> NECLGTIGPVTPLDASDFALDIRMPGVTPKESDTYFCMSMRLPVDEEAFVIDFKPRASMDTVHAMLLFGCNMPSSTGSYWFCDEGTCTDKANILYAWARNAPPTRLPKGVGFRVGGETGSKYFVLQVHYGDISAFRDNHKDCSGVSVHLTRVPQPLIAGMYLMMSVDTVIPPGEKVVNADISCQYKMYPMHVFAYRVHTHHLGKVVSGYRVRNGQWTLIGRQNPQLPQAFYPVEHPVDVTFGDILAARCVFTGEGRTEATHIGGTSSDEMCNLYIMYYMEAKYALSFMTCTKNVAPDMFRTIPAEANIPIPV

The two recently opened beamlines for macromolecular crystallography at NSLS-II have launched the microcrystallography field into new territory, with flux densities up to two orders of magnitude brighter than those previously available. In this study, we highlight the capabilities of the AMX and FMX beamlines at NSLS-II by describing structure determination from single crystal vector data collection and two methods for multicrystal data collection. The advent of next generation synchrotron beamlines has necessitated the development of new strategies to fully benefit from the increased beam intensity and smaller beam sizes while minimizing radiation damage. The high dose rates, in conjunction with the newly developed ultrafast raster scanning goniometer brings formerly time-consuming serial crystallography measurements into the minutes range. These new opportunities mean that inhomogeneous large crystals can now deliver high quality data collected from their best volume, and crystals as small as 5 to 10 µm can deliver one or more complete datasets.

PHM is a dicopper enzyme involved in peptide amidation: it hydroxylates the C-terminal glycine Cα in the first step of a sequential two-step process to produce the amidated peptide product. Amidated peptides are frequently secreted and function as hormones, neurotransmitters, and growth factors. Our lab has previously published a series of wild type and mutant PHM structures that investigate the role of copper occupancy on catalysis and substrate binding. Crystals of H108A-peptidylglycine α-hydroxylating monooxygenase (PHM) were approximately 15 × 25 × 10 µm in size. Thirteen crystals were identified in the loop and multiple centers defined for collection of partial datasets with 0.2° oscillation and a total rotation of 20° to avoid overlapping of crystals. The datasets were processed individually using XDS and seven datasets were selected and scaled with XSCALE to give a final dataset to 2.7 Å resolution with 〈I/σ(I)〉 of 2.8, with overall Rmerge of 13.0%, Rpim of 6.2%, and CC1/2 of 99.1%, with values of 58.0%, 30.9%, and 83.0% in the highest resolution shell, respectively. The structures align well, with an RMSD of only 0.6 Å. In the case of H108A-PHM, a multicentering approach was used to collect the data and then the individual datasets were processed and scaled to give a complete dataset. This option works well for cases with a handful of small, easily distinguishable crystals that will survive 10 to 20° of data collection.> MTTTMKISIEFLEPFRMTKWQESTRRNKNNKEFVRGQAFARWHRNKKDNTKGRPYITGTLLRSAVIRSAENLLTLSDGKISEKTCCPGKFDTEDKDRLLQLRQRSTLRWTDKNPCPDNAETYCPFCELLGRSGNDGKKAEKKDWRFRIHFGNLSLPGKPDFDGPKAIGSQRVLNRVDFKSGKAHDFFKAYEVDHTRFPRFEGEITIDNKVSAEARKLLCDSLKFTDRLCGALCVIRFDEYTPAADSGKQTENVQAEPNANLAEKTAEQIISILDDNKKTEYTRLLADAIRSLRRSSKLVAGLPKDHDGKDDHYLWDIGKKKKDENSVTIRQILTTSADTKELKNAGKWREFCEKLGEALYLKSKDMSGGLKITRRILGDAEFHGKPDRLEKSRSVSIGSVLKETVVCGELVAKTPFFFGAIDEDAKQTDLQVLLTPDNKYRLPRSAVRGILRRDLQTYFDSPCNAELGGRPCMCKTCRIMRGITVMDARSEYNAPPEIRHRTRINPFTGTVAEGALFNMEVAPEGIVFPFQLRYRGSEDGLPDALKTVLKWWAEGQAFMSGAASTGKGRFRMENAKYETLDLSDENQRNDYLKNWGWRDEKGLEELKKRLNSGLPEPGNYRDPKWHEINVSIEMASPFINGDPIRAAVDKRGTDVVTFVKYKAEGEEAKPVCAYKAESFRGVIRSAVARIHMEDGVPLTELTHSDCECLLCQIFGSEYEAGKIRFEDLVFESDPEPVTFDHVAIDRFTGGAADKKKFDDSPLPGSPARPLMLKGSFWIRRDVLEDEEYCKALGKALADVNNGLYPLGGKSAIGYGQVKSLGIKGDDKRISRLMNPAFDETDVAVPEKPKTDAEVRIEAEKVYYPHYFVEPHKKVEREEKPCGHQKFHEGRLTGKIRCKLITKTPLIVPDTSNDDFFRPADKEARKEKDEYHKSYAFFRLHKQIMIPGSELRGMVSSVYETVTNSCFRIFDETKRLSWRMDADHQNVLQDFLPGRVTADGKHIQKFSETARVPFYDKTQKHFDILDEQEIAGEKPVRMWVKRFIKRLSLVDPAKHPQKKQDNKWKRRKEGIATFIEQKNGSYYFNVVTNNGCTSFHLWHKPDNFDQEKLEGIQNGEKLDCWVRDSRYQKAFQEIPENDPDGWECKEGYLHVVGPSKVEFSDKKGDVINNFQGTLPSVPNDWKTIRTNDFKNRKRKNEPVFCCEDDKGNYYTMAKYCETFFFDLKENEEYEIPEKARIKYKELLRVYNNNPQAVPESVFQSRVARENVEKLKSGDLVYFKHNEKYVEDIVPVRISRTVDDRMIGKRMSADLRPCHGDWVEDGDLSALNAYPEKRLLLRHPKGLCPACRLFGTGSYKGRVRFGFASLENDPEWLIPGKNPGDPFHGGPVMLSLLERPRPTWSIPGSDNKFKVPGRKFYVHHHAWKTIKDGNHPTTGKAIEQSPNNRTVEALAGGNSFSFEIAFENLKEWELGLLIHSLQLEKGLAHKLGMAKSMGFGSVEIDVESVRLRKDWKQWRNGNSEIPNWLGKGFAKLKEWFRDELDFIENLKKLLWFPEGDQAPRVCYPMLRKKDDPNGNSGYEELKDGEFKKEDRQKKLTTPWTPWA

Cas7-11 is a Type III-E CRISPR Cas effector that confers programmable RNA cleavage and has potential applications in RNA interference. Cas7-11 encodes a single polypeptide containing four Cas7- and one Cas11-like segments that obscures the distinction between the multi-subunit Class 1 and the single-subunit Class-2 CRISPR Cas systems. The recently discovered Type III-E effector, Cas7-11 or gRAMP (for giant repeat-associated mysterious protein), is also a single subunit effector with fused Cas7-like and Cas11-like segments (van Beljouw et al., 2021; Özcan et al., 2021). Unlike Cas13 but similar to Csm/Cmr, Cas7-11 employs the Cas7-like segments to cleave crRNA-guided target RNA.

To understand the molecular basis for crRNA processing and target interference by Cas7-11, we determined a cryo-electron microscopy (cryo-EM) structure of Desulfonema ishimotonii Cas7-11 (DiCas7-11) at an overall resolution of 2.82 Å. The wild-type DiCas7-11 was incubated with its precursor crRNA (pre-crRNA) and a complementary target RNA under a reactive condition before being made frozen specimen. Under this condition, DiCas7-11 successfully processes the pre-crRNA and cleaves the target RNA. The density map resolves most of the DiCas7-11 protein, the crRNA (–15 to +19) and the partially cleaved target RNA (+19* to +2*). The core Cas7-11 assembly is half-moon shaped with four Cas7-like (C7L) domains (C7L.1–C7L.4 from N- to the C-terminus) forming a long ridge and a single Cas11-like domain (C11L) occupying the crescent center. The 34-nt crRNA lies along the C7L ridge with its repeat region spanning C7L.1-C7L.2 and the spacer region covering C7L.3-C7L.4. The first 18 nucleotides of the target RNA (+19* to +2*) remain base paired with the spacer region of the crRNA. The observed structure suggests that the pre-crRNA is processed by the first C7L domain, which yields a mature crRNA containing the last 15 nucleotides of the direct repeat (5’-tag) linked to the programmed spacer. A well-conserved histidine residue, His43, is immediately next to the leaving 5’-hydroxyl oxygen (2.3 Å) of U(–15), suggesting its role in processing. Two acidic residues, Asp429 and Asp654, were previously shown to be critical to cleavage at site 1 and site 2, respectively.> AFYKREMFDPAEKYKMDHRRRGIALIFNHERFFWHLTLPERRGTCADRDNLTRRFSDLGF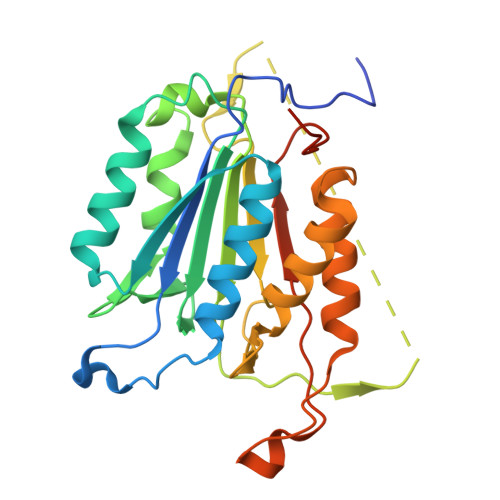EVKCFNDLKAEELLLKIHEVSTVSHADADCFVCVFLSHGEGNHIYAYDAKIEIQTLTGLFKGDKCHSLVGKPKIFIIQACRGNQHDVPVIPLDVVDAASVYTLPAGADFLMCYSVAEGYYSHRETVNGSWYIQDLCEMLGKYGSSLEFTELLTLVNRKVSQRRVDFCKDPSAIGKKQVPCFASMLTKKLHFFPKSNGNSHHHHHH The Ca2+-ATPase of sarco(endo)plasmic reticulum (SERCA) is an ion-translocating ATPase belonging to the P-type family of membrane transporters. It pumps cytosolic Ca2+ ions across the sarco- or endoplasmic reticulum (SR/ER) membrane at the expense of ATP, a vital function in all living cells, particularly in the context of muscle contraction, Ca2+ signaling, and cell survival. Binding and hydrolysis of ATP is mediated by SERCA’s cytosolic “headpiece” which consists of three roughly globular domains, the nucleotide-binding (N), phosphorylation (P), and actuator (A) domains, while the Ca2+-binding sites are located in the transmembrane (TM) part of the protein, which consists of 10 α-helices (M1 through M10). Glu340 is a centrally positioned residue in the P1 helix at the interface between the phosphorylation domain and the cytosolic ends of M3 through M7.

In this study, we have determined the crystal structure of yeast-expressed rabbit SERCA1a mutant E340A at 3.2-Å resolution in the Ca2E1 form with bound ATP analog (AMPPCP), and we examined its functional properties, including ATPase activity and Ca2+-binding kinetics. Notably, unlike other structurally characterized mutants, SERCA E340A is catalytically active, i.e., capable of completing a full catalytic cycle, albeit with altered kinetics. The E2 to Ca2E1 transition of E340A is significantly slower than that of the WT, with an increase of t1/2 of about threefold. Nevertheless, when superposed on the C-terminal transmembrane helix bundle M5 to M10 (residues 750 to 994, main chain rmsd = 0.49 Å), the E340A mutant and WT have an almost identical arrangement of the remaining transmembrane helices M1 to M4 (main chain rmsd = 0.56 Å), with a small 1.6-Å bend at the cytosolic end of M3 in E340A, and a slightly more kinked M1 helix (105° in E340A vs. 109° in WT). In line with this, the Ca2+-binding sites look identical in WT and E340A. In contrast to the almost identical arrangement in the TM domain, there is a pronounced shift (approximately 10 Å) in the position of the cytosolic headpiece, which is rotated further “downward” toward the membrane surface in E340A. Intriguingly, the downward rotation of the cytosolic headpiece in E340A is an extension of exactly the same trajectory as the movement of WT SERCA when it shifts from empty MgE1 to the Ca2+-bound E1 form (Ca2E1): when Ca2+ binds to WT SERCA, the entire P1 to M3 network moves upwards relative to L6-7 and M5, by about 4.5 Å, while the overall headpiece rotates down toward the membrane surface. While the P/N body moves as one rigid body the distance between the N and A domains increases in E340A.The main chain rmsd of 1.4 Å for the N/A body is the largest rms deviation measured for any element of the two structures, indicating that this is the largest structural change induced by the mutation.

> MEAAHSKSTEECLAYFGVSETTGLTPDQVKRHLEKYGHNELPAEEGKSLWELVIEQFEDLLVRILLLAACISFVLAWFEEGEETITAFVEPFVILLILIANAIVGVWQERNAENAIEALKEYEPEMGKVYRADRKSVQRIKARDIVPGDIVEVAVGDKVPADIRILSIKSTTLRVDQSILTGESVSVIKHTEPVPDPRAVNQDKKNMLFSGTNIAAGKALGIVATTGVSTEIGKIRDQMAATEQDKTPLQQKLDEFGEQLSKVISLICVAVWLINIGHFNDPVHGGSWIRGAIYYFKIAVALAVAAIPEGLPAVITTCLALGTRRMAKKNAIVRSLPSVATLGCTSVICSDKTGTLTTNQMSVCKMFIIDKVDGDFCSLNEFSITGSTYAPEGEVLKNDKPIRSGQFDGLVELATICALCNDSSLDFNETKGVYEKVGEATETALTTLVEKMNVFNTEVRNLSKVERANACNSVIRQLMKKEFTLEFSRDRKSMSVYCSPAKSSRAAVGNKMFVKGAPEGVIDRCNYVRVGTTRVPMTGPVKEKILSVIKEWGTGRDTLRCLALATRDTPPKREEMVLDDSSRFMEYETDLTFVGVVGMLDPPRKEVMGSIQLCRDAGIRVIMITGDNKGTAIAICRRIGIFGENEEVADRAYTGREFDDLPLAEQREACRRACCFARVEPSHKSKIVEYLQSYDEITAMTGDGVNDAPALKKAEIGIAMGSGTAVAKTASEMVLADDNFSTIVAAVEEGRAIYNNMKQFIRYLISSNVGEVVCIFLTAALGLPEALIPVQLLWVNLVTDGLPATALGFNPPDLDIMDRPPRSPKEPLISGWLFFRYMAIGGYVGAATVGAAAWWFMYAEDGPGVTYHQLTHFMQCTEDHPHFEGLDCEIFEAPEPMTMALSVLVTIEMCNALNSLSENQSLMRMPPWVNIWLLGSICLSMSLHFLILYVDPLPMIFKLKALDLTQWLMVLKISLPVIGLDEILKFIARNYLEG>HHHHHHSSGLVPRGSHMASMSKVGINGFGRIGRLVLRRLLEVKSNIDVVAINDLTSPKILAYLLKHDSNYGPFPWSVDFTEDSLIVDGKSIAVYAEKEAKNIPWKAKGAEIIVECTGFYTSAEKSQAHLDAGAKKVLISAPAGEMKTIVYNVNDDTLDGNDTIVSVASATTNCLAPMAKALHDSFGIEVGTMTTIAAYTGTQSLVDGPRGKDLRASRAAAENIIPHTTGAAKAIGLVIPELSGKLKGHAQRVPVKTGSVTELVSILGKKVTAEEVNNALKQATTNNESFGYTDEEIV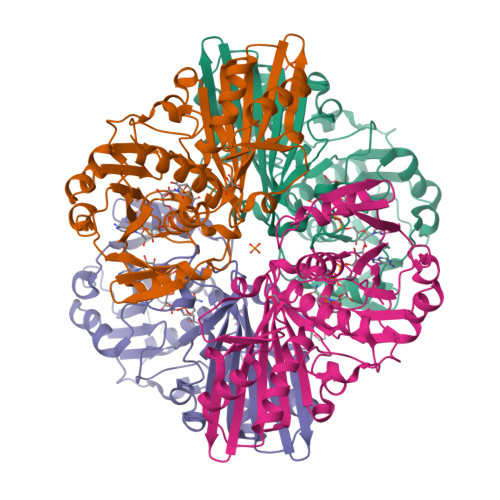SSDIIGSHFGSVFDATQTEITAVGDLQLVKTVAWYDNEYGFVTQLIRTLEKFAKL[4x]>MTSAEMTSPNNNSEHQAIAKMRTMIEGFDDISHGGLPIGRSTLVSGTSGTGKTLFSIQFLYNGIIEFDEPGVFVTFEETPQDIIKNARSFGWDLAKLVDEGKLFILDASPDPEGQEVVGGFDLSALIERINYAIQKYRARRVSIDSVTSVFQQYDASSVVRRELFRLVARLKQIGATTVMTTERIEEYGPIARYGVEEFVSDNVVILRNVLEGERRRRTLEILKLRGTSHMKGEYPFTITDHGINIFPLGAMRLTQRSSNVRVSSGVVRLDEMCGGGFFKDSIILATGATGTGKTLLVSRFVENACANKERAILFAYEESRAQLLRNAYSWGMDFEEMERQNLLKIVCAYPESAGLEDHLQIIKSEINDFKPARIAIDSLSALARGVSNNAFRQFVIGVTGYAKQEEITGLFTNTSDQFMGAHSITDSHISAITDTIILLQYVEIRGEMSRAIN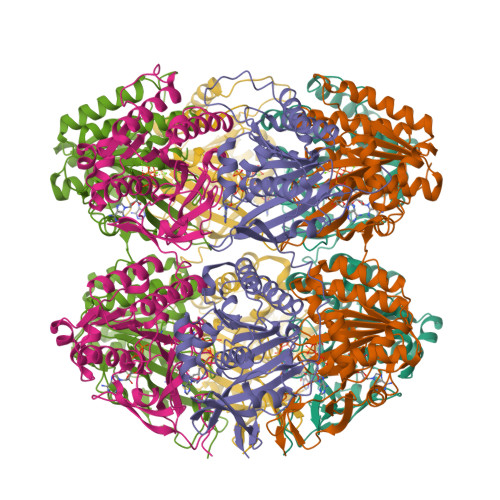VFKMRGSWHDKAIREFMISDKGPDIKDSFRNFERIISGSPTRITVDEKSELSRIVRGVQEKGPES[6x]(3S,5S)-3-({[(aminomethyl)amino]methyl}sulfanyl)-5-[(2S)-1,3-dioxobutan-2-yl]-L-proline 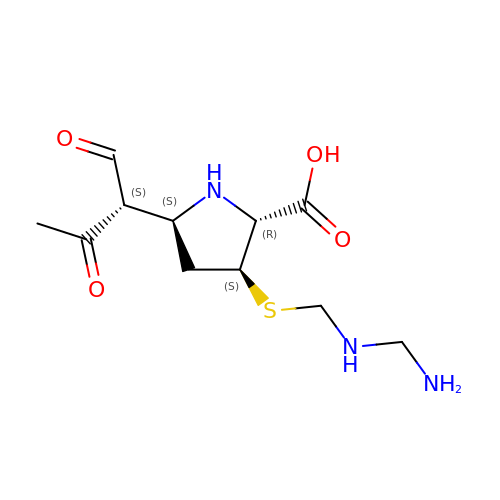| C11 H19 N3 O4 S | SKDDBJCIWUNJNL-XKNYDFJKSA-N> IDPVLEYRLSQVQSRISEERFLKNNGSGNEIGFWIFDYPAQNELQVREHLKYLLRNLEKDHKFAHLNIFQIIVDMLTERGLFDRVC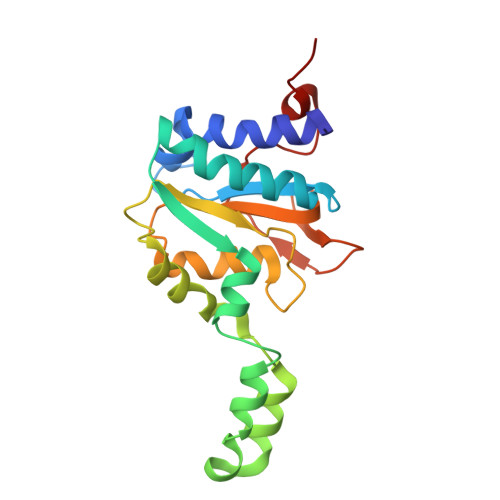QQEVKVGTEALKKQLVGLLNQKKIADYIAKKVDLQNQEFVILTGMGNAWPLVRGHELMSALQDVMGFTPLLMFYPGTYSGHDLSPLAGIDSRNYYRAFRLVPESGPAATLNPR>[2x]TYFSFWNKFSSNADINTMMLNNNADQLEPFDRADIIQDLPDFTGMNVVDVGAGIGRFTTTFAQRAKHVVSSDFIDSFIEKNKERNAAFENITYQVSDALGLQVDPQSTDLVFTNWLLMYLNEQECVRFLMKTMEWLKPGGYLHVRESCTEPSTGKSKTGSMHSDKKANPTHYRYSSVYLQLLKELRWTDARGMQWRFNVLWAKSVPTYVER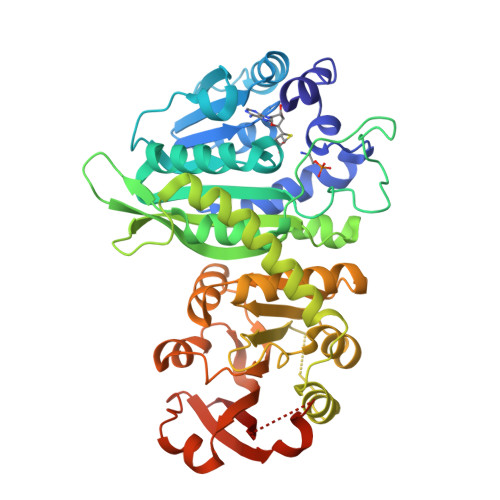VLNWRQVHWLCVKVPAQDGGISNEKALISAMGRWKIIQDHTEYLLNGKTSWATDVINNVISKVDFANNNLPLYVYSPRVVSPFVFVDSHNIAAMTGLSVWAVETNPLFYRHMLNRCVEAKDRRVQYGWNADLQSSINDWGLKKARFGGVIATELFMANSDTSLMALKEILDDNANIFTIEPALSIEDFKENVVVPENMEMIAITDVSAYVVCREQKQAFDSPNQPCWLLVHARLL>[6x]PADAVPAYPFSLPHALDLDPHYAELRRDEPVSRVRLPYGEGTAWLVTRMSDARIVLGDSRFSTAAATDPATPRMFPTPPYPDGVLAQDPPDHTRLRRLVGKAFTARRVEEMRPRVRSLVDSLLDDMVAHGSPADLVEFLAVPFPVAVICELLGVPLEDRDLFRTFSDAMLSSTRLTAAEIQRVQQDFMVYMDGLVAQRRDAPTEDLLGALALATDNDDHLTKGEIVNMGVSLLIAGHETSVNQITNLVHLLLTERKRYESLVADPALVPAAVEEMLRYTPLVSAGSFVRVATEDVELSTVTVRAGEPCVVHFASANRDEEVFDHADELDFHRERNPHIAFGHGAHHCIGAQLGRLELQEALSALVRRFPTLDLAEPVAGLKWKQGMLIRGLERQIVSW

The 8.8a-oleandolide epoxygenase OleP, from Streptomyces antibioticus, is the P450 involved in the polyketide biosynthesis of the antibiotic oleandomycin. It introduces an epoxide function to the C8-C8a of the macrolactone ring of two structurally different intermediates, namely the aglycone 8.8a-oleandolide (DEO) and the C3-mono-glycosylated L-olivosyl-8.8a-deoxyoleandolide (L-O-DEO). Substrate binding to the cytochrome P450 OleP is coupled to a large open-to-closed transition that remodels the active site, minimizing its exposure to the external solvent. When the aglycone substrate binds, a small empty cavity is formed between the I and G helices, the BC loop, and the substrate itself, where solvent molecules accumulate mediating substrate-enzyme interactions.

The tyrosine side chain at position 89 is not located inside the cavity, but it rotates towards the bulk. In the wild type OleP, the glutamate 89 was found in a double conformation, one that exposed the residue towards the solvent (flipped-out), and one towards the polar cavity (flipped-in). Therefore, the substitution with a tyrosine stabilizes the flipped-out conformation, since we found the amino acid exposed to the solvent in all of the chains identified in the asymmetric unit. The effect of this structural change is a slight increase of the volume of the catalytic pocket with respect to the wild type, which has been measured to be 671.2 Å3. In E89Y, the rotation that orients the side chain of the residue on the opposite side to the heme binding pocket eliminates the water mediated contacts established by the E89 side chain. Moreover, in E89Y, we identified one molecule of glycerol (GOL), used to cryoprotect the formed crystal, absent in the wild type, that occupies the position of the E89 sidechain and of two water molecules. Therefore, in the presence of E89Y mutation, the effect of the stabilization of the flipped-out conformation of the residue is limited to minor structural changes within the solvent cavity: (i) A slight enlargement of the cavity; (ii) the rearrangement of Q193 on G helix that rotates about 45° in the direction of the place left by the carboxyl group at the Cδ of the glutamate side chain to compensate for its absence. In this position, Q193 indirectly contacts N236 on the I helix through GOL. Furthermore, the calculation of the solvent cavity volumes as provided by MD trajectories confirms the analysis of the crystal structure, where an increase of the E89Y cavity volume with respect to the WT and G92W has been observed. Indeed, while the effect of the ionic strength on the spin state equilibrium of the wild type and E89Y is comparable, showing the total low-to-high spin shift at I = 2.5–3 M, in G92W and S240Y mutants the shift is not complete even at the highest ionic strength conditions tested (I = 3.5 M).> XQLATKAA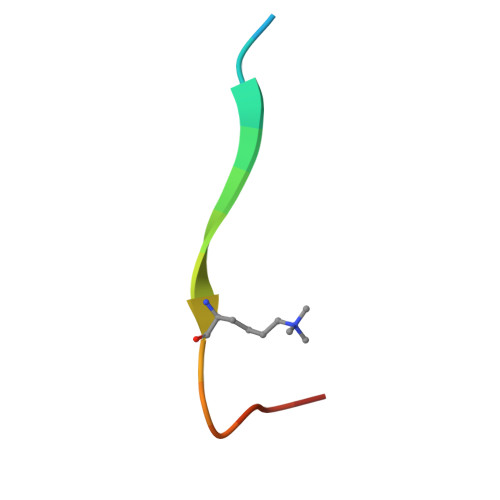RKSAPATYX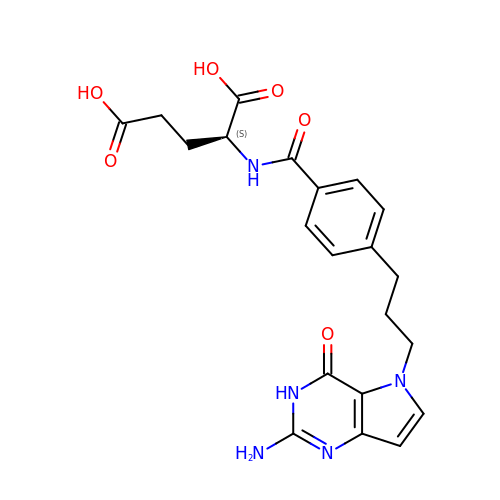N-{4-[3-(2-amino-4-oxo-3,4-dihydro-5H-pyrrolo[3,2-d]pyrimidin-5-yl)propyl]benzoyl}-L-glutamic acid | C21 H23 N5 O6 | IBENGLXKAUDADJ-HNNXBMFYSA-N Staphylococcus epidermidis expresses glycerol phosphate wall teichoic acid (WTA), but some health care–associated methicillin-resistant S. epidermidis (HA-MRSE) clones produce a second, ribitol phosphate (RboP) WTA, resembling that of the aggressive pathogen Staphylococcus aureus. We report here that the TarM enzyme of HA-MRSE [TarM(Se)] glycosylates RboP-WTA with glucose, instead of N-acetylglucosamine (GlcNAc) by TarM(Sa) in S. aureus. Each blade of the homotrimer contains a catalytic domain with a canonical GT-B fold, consisting of an N-terminal acceptor substrate-binding domain (ABD; residues 1 to 68 and 202 to 302) and a C-terminal nucleotide-binding domain (residues 303 to 492). TarM(Se) is a retaining WTA glycosyltransferase; therefore, the relative positions of donor and acceptor substrates in TarM(Se) and TarP are different.

The ribitol moiety of RboP1 forms three hydrogen bonds with the side chains of Asn9 and Gln265, as well as the backbone carbonyl group of Gly229. Three main-chain amide groups interact with the phosphate group of RboP2. Two of these are from tandem backbone amide groups of Gly229 and Ser230, and the third one is contributed by Asn9; this phosphate group is also hydrogen-bonded to the side chain of Ser230. The ribitol moiety of RboP2 has only contact with the side chain and backbone amide group of Glu10. The phosphate group of RboP3 interacts with tandem backbone amide groups of Met18 and Thr19 and is further hydrogen-bonded to the Thr19 side chain. We could not find any electron density for the ribitol moiety of RboP3, the entire RboP4 unit, and the linker region of the molecule. The interactions between RboP1 and TarM(Se)G117R are all conserved as in the binary structure.

>[4x]MHHHHHHSGENLYFQSMKQTYMIVNELDVNKGGMTTAMLTRSKFFLDNEISGDIITFDFKANYKDILKELVQSKKMDKRTQMHNPFIYFKNISNLQHKKYNYTMTRNLSNLLKDSVEIKENSRISRFFNIMSREYLAYKRETEQETIFDLFKNNLRYKRIYFYKGKIVKTEVFNSDNNLIAEQFYDDNGYLYLYRQINPEKKSIGKTYLVCKEKQFKNNVEFCSYFLDKLIPDINDNIIICDGPGSFPKILKTNHKNVKKFAVIHVNHYKNFDDTGAVKKQEDYILRNANKINGVVMLTEAQKKDIIEKYKITNAYVISNFINITDDYRDKNDNKVVGHISRLVPQKGLPYLIDVAKKVVEQDNSVEFHLYGTGEEKSKIENLIQESNLTNNVKLLGYTTNAIEKIKDFRCVISTSQFEGQGLSLIEAMLLKKPVVAFDVKYGPSDFVKDGKNGYLIENKDIKKMANKILKLLHDKELSKSLGKHGRDTIIDMYQPEKLMVKWKQLFN>[4x]MSLRQVIPIPSPPAKYLLPEVTVLDYGKKCVVIDLDETLVHSSFKPISNADFIVPVEIDGTIHQVYVLKRPHVDEFLQRMGQLFECVLFTASLAKYADPVADLLDR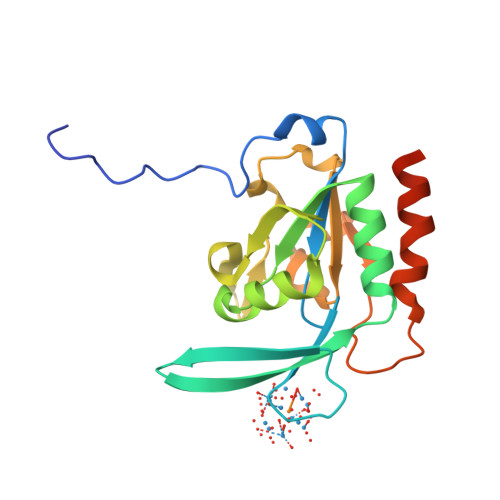WGVFRARLFRESCVFHRGNYVKDLSRLGRELSKVIIVDNSPASYIFHPENAVPVQSWFDDMTDTELLDLIPFFEGLSREDDEGHHHHHH> SQFERGYTSPYFVTDPERMICEYENCKILLVDKKISTARDIITILESAIRGNYPLLIMAEEVEQEALATLVVNKLRGTLKVVAIKAPGFGERRSSYLEDIAILTGGTVVRDEMGVSLEQATDAVLGTAAKITITKERTTVVGDGSTAADVAARVKQIRNLQMQTDQDY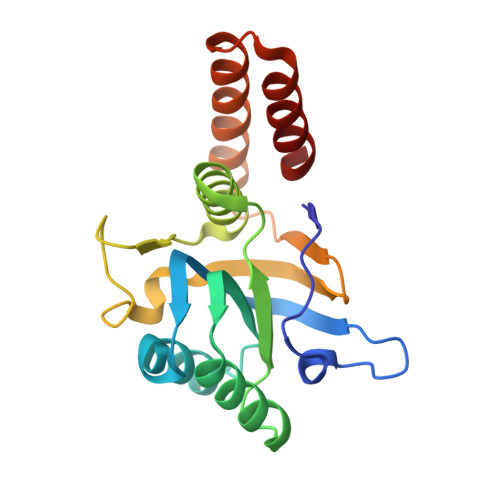EREKLQERIARLSGG> GPMPGKKFVARVAEAGGKRVVIIPKAERAKVGIKVGDVVEVKKV

Here, we study fold transition between distinct β-barrels by protein engineering and structural biology technique. Here, we discover that the previously reconstructed ancient DPBB sequence could also adopt a β-barrel fold named Double-Zeta β-barrel (DZBB), as a metamorphic protein. The DZBB fold is not found in any modern protein, although its structure shares similarities with RIFT and OB. Furthermore, the reconstructed OB fold could also be converted to the four-stranded SH3 fold by a simple circular permutation. Thus, these ancient β-barrel folds (DPBB, RIFT, OB, and SH3) could be readily interconverted by a few feasible mutations through the missing-link fold, DZBB, indicating their significantly close evolutionary relationships.

In contrast, design-4 was unfolded but still formed crystals in the presence of sulfate ions. The crystallographic analysis revealed that design-3 and design-4 adopted the homo-dimeric RIFT-fold. Thus, the short In/Del at the 1st loop position is the determinant for the fold transition between DZBB and RIFT. A single deletion in the DZBB sequence converted it into the RIFT fold. Most DNA molecules did not migrate from the well when mixed with the proteins with the stable DZBB fold (design-2, -18, and -19) and RIFT fold (design-3 and -4), indicating that these proteins formed large aggregates with dsDNA. In particular, design-2, -18, -19, -3, and -4 interacted with dsDNA even in high salt conditions (500 mM NaCl).> GS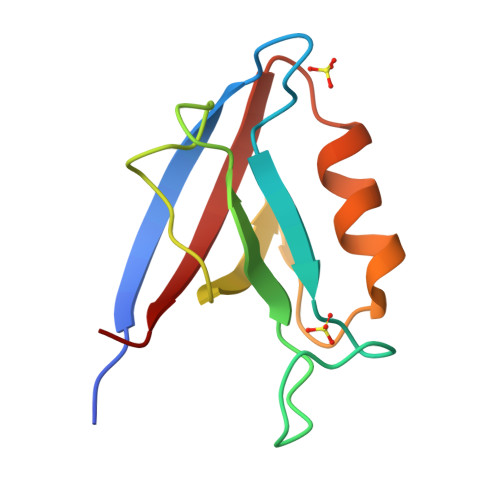HMIWEQHTVTLHRAPGFGFGIAISGGRDNPHFQSGETSIVISDVLKGGPAEGQLQENDRVAMVNGVSMDNVEHAFAVQQLRKSGKNAKITIRRKK> SFLSNVKYNFMRIIKYEFILNDALNQSIIRANAQYLTAAALHNLDEAVKFDMGAYKSSKDDAKITVILRISKTQLYVTAQDEDQPVLLKEMPEIPKTIT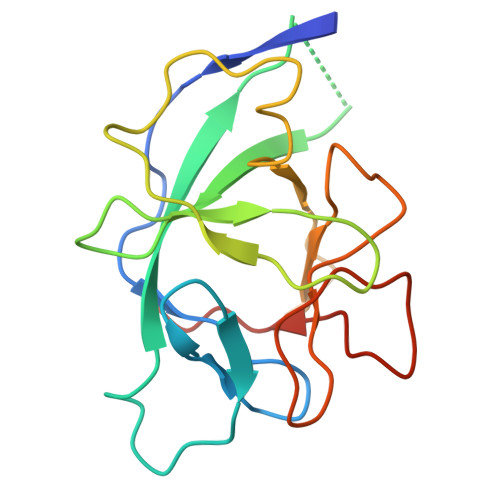GSETNLLFFWETHGTKNYFTSVAHPNLFIATKQDYWVCLAGGPPSITDFQILENQA>[2x]MVSTAPYGAWQSPIDAALVASRSGRPACVGA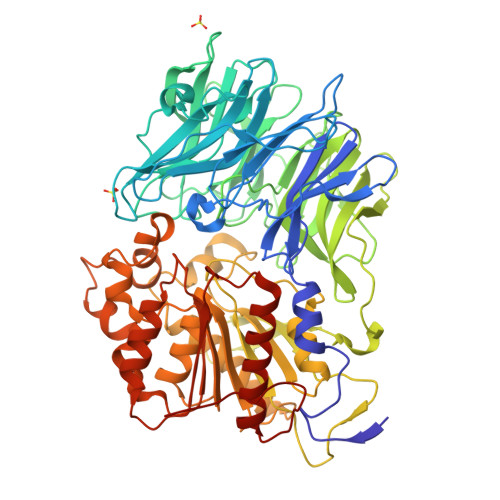VGDEVWWVAPRPAEAGRATLVRRRADGAEESALPAPWNVRNRVFEYSGFPWAGVPRPAGGPLLVFTHFGDQRLYAFEPDAPGGAVPRPLTPVSAVGGGLRWADPVLLPERGEVWCMAEEFTGEGPSDVRRFLAAVPLDGSAAADRSAVRELSDDAHRFVTGPRLSPDGRQAVWLAWDHPRMPWEGTELKTARVTEDGRFADTRTLLGGPEEAIAQAEWAPDGSLIVATDRTGWWNLHRVDPATGAATQLCRREEEFAGPLWTPGMRWFAPLANGLIAVVHGKGAAVLGILDPESGELVDAAGPWTEWAATLTVSGTRAVGVAASPRTAYEVVELDTVTGRARTIGARHTDPVDPAYYPEPQIRTFTAPDGREIHAHIYPPHSPDFTGPADELPPYVVMAHGGPTSRVPAVLDLDVAYFTSRGIGVADVNYGGSTGYGRAYRERLRGRWGVVDVEDCAAVATALAEEGTADRARLAVRGGAAGGWTAASSLVSTDVYACGTVLYPVLDLLGWADGGTHDFESRYLDFLIGSFEEFPERYRDRAPLTRADRVRVPFLLLQGLEDPVCPPEQCDRFLEAVAGCGVPHAYLSFEGEGHGFRRKETMVRALEAELSLYAQVFGVEVAGVPLLKLGE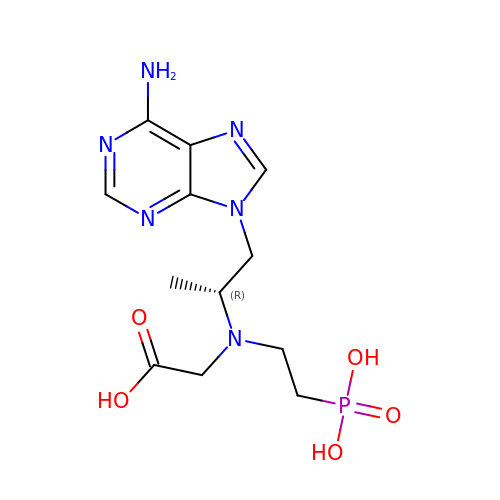(R)-N-(1-(6-amino-9H-purin-9-yl)propan-2-yl)-N-(2-phosphonoethyl)glycine | C12 H19 N6 O5 P | KATXUXXXPKCCGG-MRVPVSSYSA-N>[2x]MVMGKRHMQQQWSAVDNY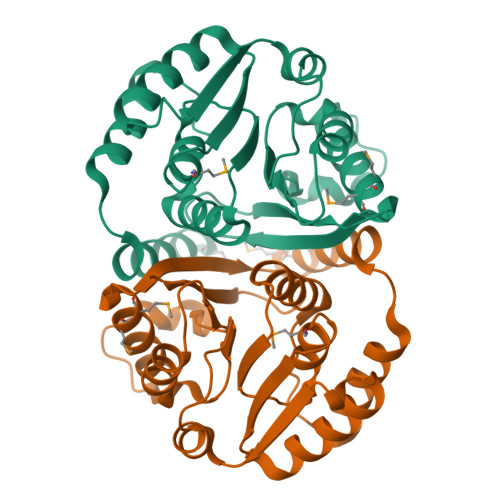LIKALIPGDPVLDRVLENNHRAGLPAHDVAANQGQFLALLVRLTQAKRILEIGTLGGYSTIWMARELPADGQLLTLEADAHHAQVARENLQLAGVDQRVTLREGPALQSLESLGECPAFDLIFIDADKPNNPHYLRWALRYSRPGTLIIGDNVVRDGEVVNPQSADERVQGVRQFIEMMGAEPRLTATALQTVGTKGWDGFTLAWVNAAENLYFQSHHHHHHWSHPQFEK>MAGKKVLIVYAHQEPKSFNGSLKNVAVDELSRQG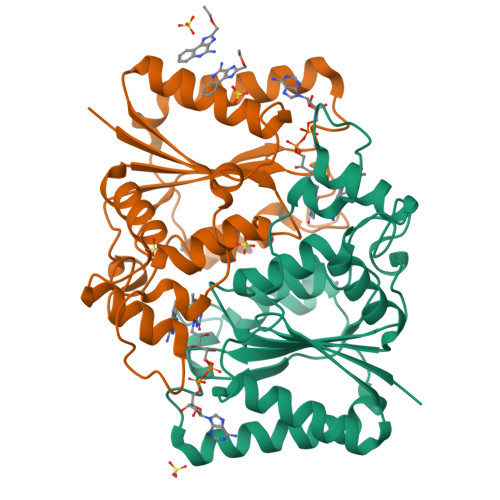CTVTVSDLYAMNLEPRATDKDITGTLSNPEVFNYGVETHEAYKQRSLASDITDEQKKVREADLVIFQFPLYWFSVPAILKGWMDRVLCQGFAFDIPGFYDSGLLQGKLALLSVTTGGTAEMYTKTGVNGDSRYFLWPLQHGTLHFCGFKVLAPQISFAPEIASEEERKGMVAAWSQRLQTIWKEEPIPCTAHWHFGQHHHHHH[2x]>[2x]GSHMRFDEFGNIITDSAVAEEPEPELPGVTEEALRLKEAALEELAAQEVTAPLVPLAVSAFLTSRKKAAAAELADWMQSPEGQASSLESIGRSLSRRNHGRSRAVVLAHDHDEAIKGLRAVAAGKQAPNVFSVDGPVTTGPVWVLAGFGAQHRKMGKSLYLR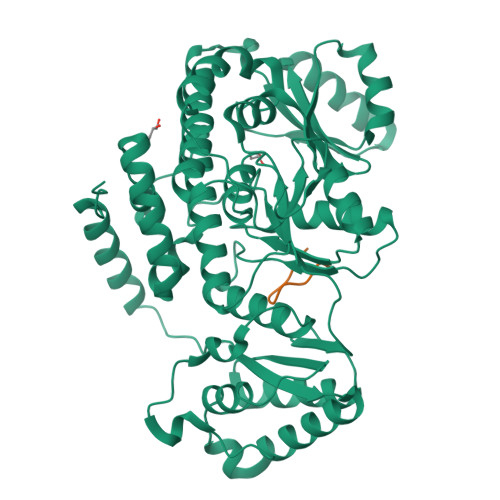NEVFAAWIEKVDALVQDELGYSVLELILDDAQDYGIETTQVTIFAIQIALGELLRHHGAKPAAVIGQSLGEAASAYFAGGLSLRDATRAICSRSHLMGEGEAMLFGEYIRLMALVEYSADEIREVFSDFPDLEVCVYAAPTQTVIGGPPEQVDAILARAEAEGKFARKFATKGASHTSQMDPLLGELTAELQGIKPTSPTCGIFSTVHEGRYIKPGGEPIHDVEYWKKGLRHSVYFTHGIRNAVDSGHTTFLELAPNPVALMQVALTTADAGLHDAQLIPTLARKQDEVSSMVSTMAQLYVYGHDLDIRTLFSRASGPQDYANIPPTRF;>[2x]SDKENFWGMAVA ethyl ~{N}-[2-(1,3-benzothiazol-2-ylcarbonylamino)-5-fluoranyl-thiophen-3-yl]carbonylcarbamate 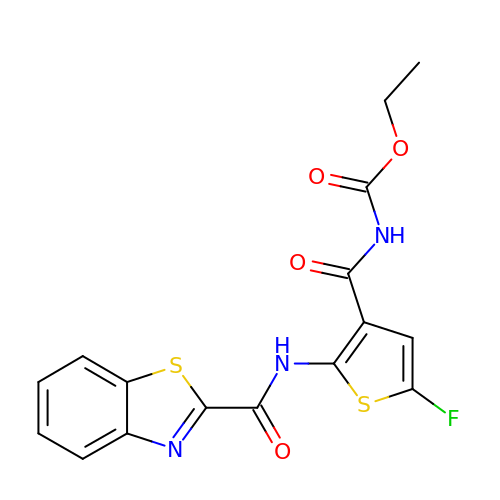| C16 H12 F N3 O4 S2 | QMDPRTOSNLYXIQ-UHFFFAOYSA-N>[4x]CCGGAGGAA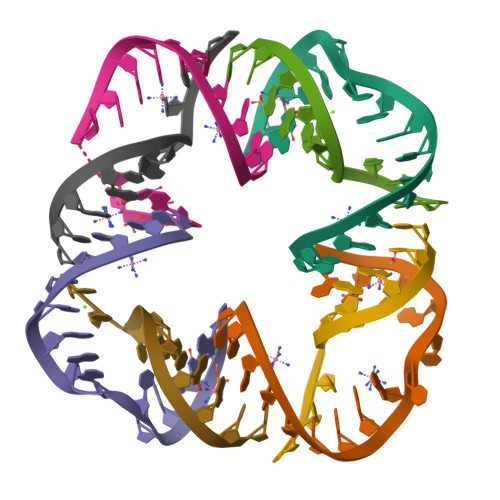CUACUG;>CCGGCAGCCU[4x]> VDIAAFDPDKDGTIDLKEALAAGSAAFDKLDPDKDGTLDAKELKGRVSEADLKKLDPDNDGTLDKKEYLAAVEAQFKAANPDNDGTIDARELASPAGSALVNLIR

The discovery of the founding member of the LanM family of lanthanide-binding proteins demonstrated that nature has evolved macromolecules surpassing the selectivity of synthetic f-element chelators. The natural lanthanide-binding protein lanmodulin (LanM)4,5 is a sustainable alternative to conventional solvent-extraction-based separation. First, LanMs possess four EF-hand motifs. Second, adjacent EF hands in LanMs are separated by 12–13 residues—rather than the typical ≈25 residues in CaII-responsive EF-hand proteins—resulting in an unusual three-helix bundle architecture with the metal-binding sites on the periphery.

Finally, we report a 1.01-Å-resolution structure of NdIII–Mex-LanM, which rationalizes Mex-LanM’s shallower RE selectivity trend. EF hands comprise 12-residue, carboxylate-rich metal-binding loops flanked by α-helices, which traditionally respond to CaII binding;29 in Mex-LanM, however, EF hands 1–3 bind lanthanide(III) ions with low-picomolar affinity and 108-fold selectivity over CaII, resulting in a large, lanthanide-selective disorder-to-order conformational transition. EF4 binds with only micromolar affinity. Unusually among RE chelators, Mex-LanM favours the larger and more abundant light REs (LREs), especially LaIII–SmIII, over heavy REs (HREs). The metal-binding sites of Mex-LanM differ substantially from those of Hans-LanM. Although the NdIII sites of Mex-LanM share the nine- and ten-coordination observed in DyIII– and LaIII–Hans-LanM, they structurally resemble the seven-coordinate CaII-binding sites of calmodulin. The increased coordination numbers in Mex-LanM relative to calmodulin result from bidentate coordination of D5 and an additional solvent ligand. The observation of the two solvent molecules per metal site and the hydrogen bond to the D9 residue validates recent spectroscopic studies.> NCYNKFAHIYDKLIRADVDYKKWSDFIIEKCVENNLVFDDYLDLACGTGNLTENL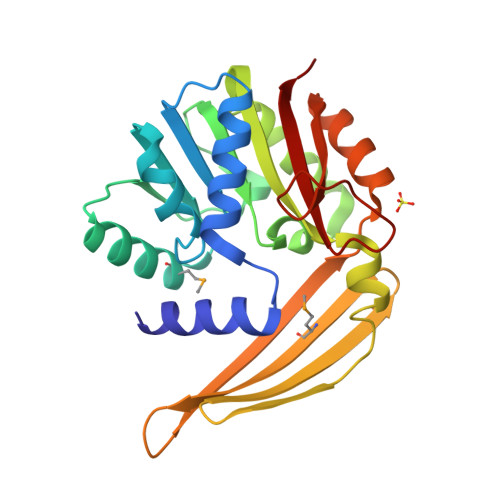CPKFKNTWAVDLSQEMLSEAENKFRSQGLKPRLACQDISNLNINRKFDLITCCLDSTNYIIDSDDLKKYFKAVSNHLKEGGVFIFDINSYYKLSQVLGNNDFNYDDDEVFYYWENQFEDDLVSMYISFFVRDGEFYKRFDEEHEERAYKEEDIEKYLKHGQLNILDKVDCYSNKKVEKFTERITYLVKLGG>[5x]MNESVKEIPDVLKSQCGFNCLTDISHSSFNEFRQQVSEHLSWSETHDLYHDAQQAQKDNRLYEARILKRANPQLQNAVHLAILAPNAELIGYNNQFSGRASQYVAPGTVSSMFSPAAYLTELYREARNLHASDSVYYLDTRRPDLKSMALSQQNMDIELSTLSLSNELLLESIKTESKLENYTKVMEMLSTFRPSGATPYHDAYENVREVIQLQDPGLEQLNASPAIAGLMHQASLLGINASISPELFNILTEEITEGNAEELYKKNFGNIEPASLAMPEYLKRYYNLSDEELSQFIGKASNFGQQEYSNNQLITPVVNSSDGTVKVYRITREYTTNAYQMDVELFPFGGENYRLDYKFKNFYNASYLSIKLNDKRELVRTEGAPQVNIEYSANITLNTADISQPFEIGLTRVLPSGSWAYAAAKFTVEEYNQYSFLLKLNKAIRLSRATELSPTILEGIVRSVNLQLDINTDVLGKVFLTKYYMQRYAIHAETALILCNAPISQRSYDNQPSQFDRLFNTPLLNGQYFSTGDEEIDLNSGSTGDWRKTILKRAFNIDDVSLFRLLKITDHDNKDGKIKNNLKNLSNLYIGKLLADIHQLTIDELDLLLIAVGEGKTNLSAISDKQLATLIRKLNTITSWLHTQKWSVFQLFIMTSTSYNKTLTPEIKNLLDTVYHGLQGFDKDKADLLHVMAPYIAATLQLSSENVAHSVLLWADKLQPGDGAMTAEKFWDWLNTKYTPGSSEAVETQEHIVQYCQALAQLEMVYHSTGINENAFRLFVTKPEMFGAATGAAPAHDALSLIMLTRFADWVNALGEKASSVLAAFEANSLTAEQLADAMNLDANLLLQASIQAQNHQHLPPVTPENAFSCWTSINTILQWVNVAQQLNVAPQGVSALVGLDYIQSMKETPTYAQWENAAGVLTAGLNSQQANTLHAFLDESRSAALSTYYIRQVAKAAAAIKSRDDLYQYLLIDNQVSAAIKTTRIAEAIASIQLYVNRALENVEENANSGVISRQFFIDWDKYNKRYSTWAGVSQLVYYPENYIDPTM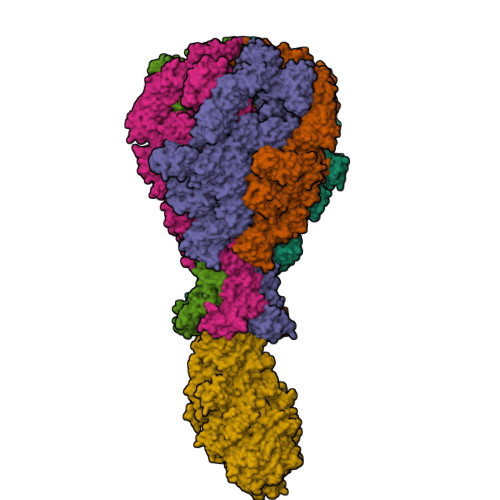RIGQTKMMDALLQSVSQSQLNADTVEDAFMSYLTSFEQVANLKVISAYHDNINNDQGLTYFIGLSETDAGEYYWRSVDHSKFNDGKFAANAWSEWHKIDCPINPYKSTIRPVIYKSRLYLLWLEQKEITKQTGNSKDGYQTETDYRYELKLAHIRYDGTWNTPITFDVNKKISELKLEKNRAPGLYCAGYQGEDTLLVMFYNQQDTLDSYKNASMQGLYIFADMASKDMTPEQSNVYRDNSYQQFDTNNVRRVNNRYAEDYEIPSSVSSRKDYGWGDYYLSMVYNGDIPTINYKAASSDLKIYISPKLRIIHNGYEGQKRNQCNLMNKYGKLGDKFIVYTSLGVNPNNSSNKLMFYPVYQYSGNTSGLNQGRLLFHRDTTYPSKVEAWIPGAKRSLTNQNAAIGDDYATDSLNKPDDLKQYIFMTDSKGTATDVSGPVEINTAISPAKVQIIVKAGGKEQTFTADKDVSIQPSPSFDEMNYQFNALEIDGSGLNFINNSASIDVTFTAFAEDGRKLGYESFSIPVTLKVSTDNALTLHHNENGAQYMQWQSYRTRLNTLFARQLVARATTGIDTILSMETQNIQEPQLGKGFYATFVIPPYNLSTHGDERWFKLYIKHVVDNNSHIIYSGQLTDTNINITLFIPLDDVPLNQDYHAKVYMTFKKSPSDGTWWGPHFVRDDKGIVTINPKSILTHFESVNVLNNISSEPMDFSGANSLYFWELFYYTPMLVAQRLLHEQNFDEANRWLKYVWSPSGYIVHGQIQNYQWNVRPLLEDTSWNSDPLDSVDPDAVAQHDPMHYKVSTFMRTLDLLIARGDHAYRQLERDTLNEAKMWYMQALHLLGDKPYLPLSTTWSDPRLDRAADITTQNAHDSAIVALRQNIPTPAPLSLRSANTLTDLFLPQINEVMMNYWQTLAQRVYNLRHNLSIDGQPLYLPIYATPADPKALLSAAVATSQGGGKLPESFMSLWRFPHMLENARGMVSQLTQFGSTLQNIIERQDAEALNALLQNQAAELILTNLSIQDKTIEELDAEKTVLEKSKAGAQSRFDSYGKLYDENINAGENQAMTLRASAAGLTTAVQASRLAGAAADLVPNIFGFAGGGSRWGAIAEATGYVMEFSANVMNTEADKISQSETYRRRRQEWEIQRNNAEAELKQIDAQLKSLAVRREAAVLQKTSLKTQQEQTQSQLAFLQRKFSNQALYNWLRGRLAAIYFQFYDLAVARCLMAEQAYRWELNDDSARFIKPGAWQGTYAGLLAGETLMLSLAQMEDAHLKRDKRALEVERTVSLAEVYAGLPKDNGPFSLAQEIDKLVSQGSGSAGSGNNNLAFGAGTDTKTSLQASVSFADLKIREDYPASLGKIRRIKQISVTLPALLGPYQDVQAILSYGDKAGLANGCEALAVSHGMNDSGQFQLDFNDGKFLPFEGIAIDQGTLTLSFPNASMPEKGKQATMLKTLNDIILHIRYTIK;> MQNSQDFSITELSLPKGGGAITGMGEALTPTGPDGMAALSLPLPISAGRGYAPAFTLNYNSGAGNSPFGLGWDCNVMTIRRRTHFGVPHYDETDTFLGPEGEVLVVADQPRDESTLQGINLGATFTVTGYRSRLESHFSRLEYWQPKTTGKTDFWLIYSPDGQVHLLGKSPQARISNPSQTTQTAQWLLEASVSSRGEQIYYQYRAEDDTGCEADEITHHLQATAQRYLHIVYYGNRTASETLPGLDGSAPSQADWLFYLVFDYGERSNNLKTPPAFSTTGSWLCRQDRFSRYEYGFEIRTRRLCRQVLMYHHLQALDSKITEHNGPTLVSRLILNYDESAIASTLVFVRRVGHEQDGNVVTLPPLELAYQDFSPRHHAHWQPMDVLANFNAIQRWQLVDLKGEGLPGLLYQDKGAWWYRSAQRLGEIGSDAVTWEKMQPLSVIPSLQSNASLVDINGDGQLDWVITGPGLRGYHSQRPDGSWTRFTPLNALPVEYTHPRAQLADLMGAGLSDLVLIGPKSVRLYANTRDGFAKGKDVVQSGDITLPVPGADPRKLVAFSDVLGSGQAHLVEVSATKVTCWPNLGRGRFGQPITLPGFSQPATEFNPAQVYLADLDGSGPTDLIYVHTNRLDIFLNKSGNGFAEPVTLRFPEGLRFDHTCQLQMADVQGLGVASLILSVPHMSPHHWRCDLTNMKPWLLNEMNNNMGVHHTLRYRSSSQFWLDEKAAALTTGQTPVCYLPFPIHTLWQTETEDEISGNKLVTTLRYARGAWDGREREFRGFGYVEQTDSHQLAQGNAPERTPPALTKNWYATGLPVIDNALSTEYWRDDQAFAGFSPRFTTWQDNKDVPLTPEDDNSRYWFNRALKGQLLRSELYGLDDSTNKHVPYTVTEFRSQVRRLQHTDSRYPVLWSSVVESRNYHYERIASDPQCSQNITLSSDRFGQPLKQLSVQYPRRQQPAINLYPDTLPDKLLANSYDDQQRQLRLTYQQSSWHHLTNNTVRVLGLPDSTRSDIFTYGAENVPAGGLNLELLSDKNSLIADDKPREYLGQQKTAYTDGQNTTPLQTPTRQALIAFTETTVFNQSTLSAFNGSIPSDKLSTTLEQAGYQQTNYLFPRTGEDKVWVAHHGYTDYGTAAQFWRPQKQSNTQLTGKITLIWDANYCVVVQTRDAAGLTTSAKYDWRFLTPVQLTDINDNQHLITLDALGRPITLRFWGTENGKMTGYSSPEKASFSPPSDVNAAIELKKPLPVAQCQVYAPESWMPVLSQKTFNRLAEQDWQKLYNARIITEDGRICTLAYRRWVQSQKAIPQLISLLNNGPRLPPHSLTLTTDRYDHDPEQQIRQQVVFSDGFGRLLQAAARHEAGMARQRNEDGSLIINVQHTENRWAVTGRTEYDNKGQPIRTYQPYFLNDWRYVSNDSARQEKEAYADTHVYDPIGREIKVITAKGWFRRTLFTPWFTVNEDENDTAAEVKKVKMMKNIDPKLYQKTPTVSVYDNRGLIIRNIDFHRTTANGDPDTRITRHQYDIHGHLNQSIDPRLYEAKQTNNTIKPNFLWQYDLTGNPLCTESIDAGRTVTLNDIEGRPLLTVTATGVIQTRQYETSSLPGRLLSVAEQTPEEKTSRITERLIWAGNTEAEKDHNLAGQCVRHYDTAGVTRLESLSLTGTVLSQSSQLLIDTQEANWTGDNETVWQNMLADDIYTTLSTFDATGALLTQTDAKGNIQRLAYDVAGQLNGSWLTLKGQTEQVIIKSLTYSAAGQKLREEHGNDVITEYSYEPETQRLIGIKTRRPSDTKVLQDLRYEYDPVGNVISIRNDAEATRFWHNQKVMPENTYTYDSLYQLISATGREMANIGQQSHQFPSPALPSDNNTYTNYTRTYTYDRGGNLTKIQHSSPATQNNYTTNITVSNRSNRAVLSTLTEDPAQVDALFDAGGHQNTLISGQNLNWNTRGELQQVTLVKRDKGANDDREWYRYSGDGRRMLKINEQQASNNAQTQRVTYLPNLELRLTQNSTATTEDLQVITVGEAGRAQVRVLHWESGKPEDIDNNQLRYSYDNLIGSSQLELDSEGQIISEEEYYPYGGTALWAARNQTEASYKTIRYSGKERDATGLYYYGYRYYQPWIGRWLSSDPAGTIDGLNLYRMVRNNPVTLLDPDGLMPTIAERIAALKKNKVTDSAPSPANATNVAINIRPPVAPKPSLPKASTSSQPTTHPIGAANIKPTTSGSSIVAPLSPVGNKSTSEISLPESAQSSSSSTTSTNLQKKSFTLYRADNRSFEEMQSKFPEGFKAWTPLDTKMARQFASIFIGQKDTSNLPKETVKNISTWGAKPKLKDLSNYIKYTKDKSTVWVSTAINTEAGGQSSGAPLHKIDMDLYEFAIDGQKLNPLPEGRTKNMVPSLLLDTPQIETSSIIALNHGPVNDAEISFLTTIPLKNVKPHKR> AYGIGLDITELKRIASMAGRQKRFAERILTRSELDQYYELSEARKNEFLAGRFAAKEAFSKAFGTGIGRQLSFQDIEIRKDQNGKPYIICTKLSQAAVHVSITHTKEYAAAQVV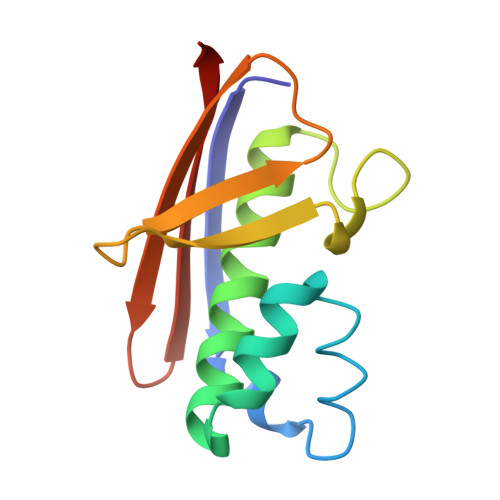IERLSS> MNHSLKPWNTFGIDHNAQHIVCAEDEQQLLNAWQYATAEGQPVLILGEGSNVLFLEDYRGTVIINRIKGIEIHDEPDAWYLHVGAGENWHRLVKYTLQEGMPGLENLALIPGCVGSSPIQNIGAYGVELQRVCAYVDSVELATGKQVRLTAKECRF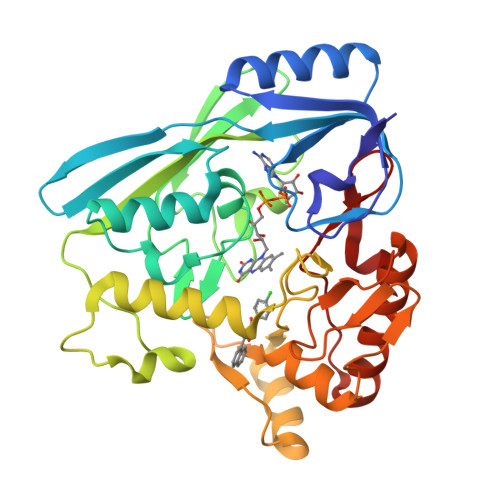GYRDSIFKHEYQDRFAIVAVGLRLPKEWQPVLTYGDLTRLDPTTVTPQQVFNAVCHMRTTKLPDPKVNGNAGSFFKNPVVSAETAKALLSQFPTAPNYPQADGSVKLAAGWLIDQCQLKGMQIGGAAVHRQQALVLINEDNAKSEDVVQLAHHVRQKVGEKFNVWLEPEVRFIGASGEVSAVETIS>MAEKPKLHYFNARGRMESTRWLLAAAGVEFEEKFIKSAEDLDKLRNDGYLMFQQVPMVEIDGMKLVQTRAILNYIASKYNLYGKDIKERALIDMYIEGIADLGEMILLLPVCPPEEKDAKLALIKEKIKNRYFPAFEKVLKSHGQDYLVGNKLSRADIHLVELLYYVEELDSSLISSFPLLKALKTRISNLPTVKKFLQPGSPRKPPMD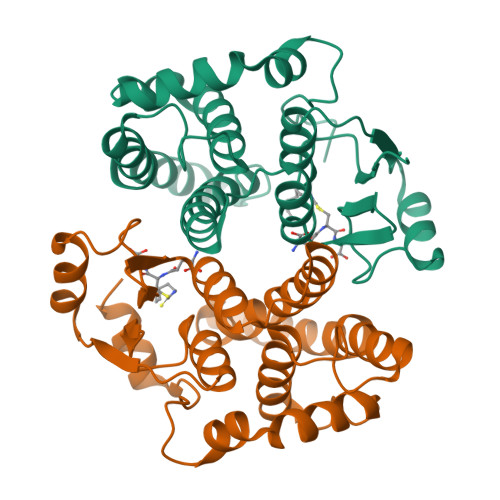EKSLEEARKIFRF[2x]> MSKFLDRFRYFKQKGETFADGHGQLLNTNRDWEDGYRQRWQHDKIVRSTSGVNCTGSCSWKIYVKNGLVTWETQQTDYPRTRPDLPNHEPRGCPRGASYSWYLYSANRLKYPMMRKRLMKMWREAKALHSDPVEAWASIIEDADKAKSFKQARGRGGFVRSSWQEVNELIAASNVYTIKNYGPDRVAGFSPIPAMSMVSYASGARYLSLIGGTCLSFYDWYCDLPPASPQTWGEQTDVPESADWYNSSYIIAWGSNVPQTRTPDAHFFTEVRYKGTKTVAVTPDYAEIAKLCDLWLAPKQGTDAAMALAMGHVMLREFHLDNPSQYFTDYVRRYTDMPMLVMLEERDGYYAAGRMLRAADLVDALG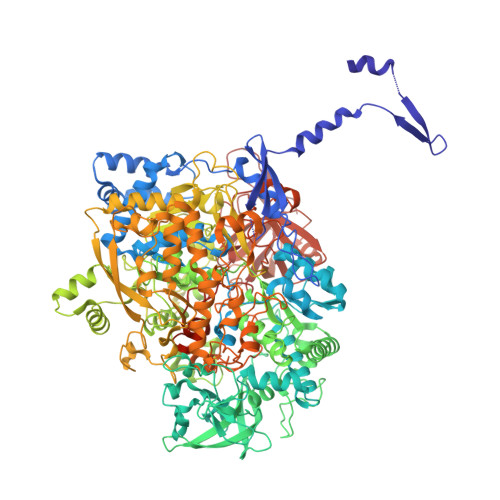QENNPEWKTVAFNTNGEMVAPNGSIGFRWGEKGKWNLEQRDGKTGEETELQLSLLGSQDEIAEVGFPYFGGDGTEHFNKVELENVLLHKLPVKRLQLADGSTALVTTVYDLTLANYGLERGLNDVNCATSYDDVKAYTPAWAEQITGVSRSQIIRIAREFADNADKTHGRSMIIVGAGLNHWYHLDMNYRGLINMLIFCGCVGQSGGGWAHYVGQEKLRPQTGWQPLAFALDWQRPARHMNSTSYFYNHSSQWRYETVTAEELLSPMADKSRYTGHLIDFNVRAERMGWLPSAPQLGTNPLTIAGEAEKAGMNPVDYTVKSLKEGSIRFAAEQPENGKNHPRNLFIWRSNLLGSSGKGHEFMLKYLLGTEHGIQGKDLGQQGGVKPEEVDWQDNGLEGKLDLVVTLDFRLSSTCLYSDIILPTATWYEKDDMNTSDMHPFIHPLSAAVDPAWEAKSDWEIYKAIAKKFSEVCVGHLGKETDIVTLPIQHDSAAELAQPLDVKDWKKGECDLIPGKTAPHIMVVERDYPATYERFTSIGPLMEKIGNGGKGIAWNTQSEMDLLRKLNYTKAEGPAKGQPMLNTAIDAAEMILTLAPETNGQVAVKAWAALSEFTGRDHTHLALNKEDEKIRFRDIQAQPRKIISSPTWSGLEDEHVSYNAGYTNVHELIPWRTLSGRQQLYQDHQWMRDFGESLLVYRPPIDTRSVKEVIGQKSNGNQEKALNFLTPHQKWGIHSTYSDNLLMLTLGRGGPVVWLSEADAKDLGIADNDWIEVFNSNGALTARAVVSQRVPAGMTMMYHAQERIVNLPGSEITQQRGGIHNSVTRITPKPTHMIGGYAHLAYGFNYYGTVGSNRDEFVVVRKMKNIDWLDGEGNDQVQESVK(2~{S},3~{R},4~{S})-2-[(2~{S},3~{R})-1,3-bis(oxidanyl)-1-oxidanylidene-butan-2-yl]-4-[(3~{S},5~{S})-5-(dimethylcarbamoyl)pyrrolidin-3-yl]sulfanyl-3-methyl-3,4-dihydro-2~{H}-pyrrole-5-carboxylic 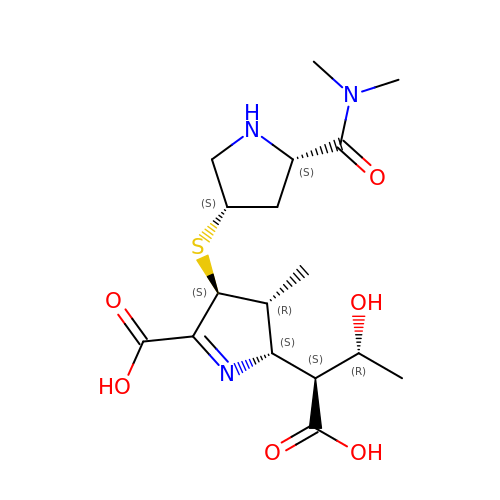acid | C17 H27 N3 O6 S | CDYPSIIDXKMBLV-CFINEGTKSA-N NAs are also present in other biological systems, for example bacteria, and these non-influenza NAs are critical virulence factors in many pathogenic organisms including Streptococcus pneumoniae, Pseudomonas aeruginosa, and Vibrio cholerae. The viral enzyme is a mushroom-like shaped homotetramer, while the bacterial NA is a monomer with two flanking lectin-like domains. Both enzymes share the canonical six-blade β-propeller fold of the catalytic NA domain, despite exhibiting a relatively low amino acid sequence identity of only 12% as revealed by structure-based sequence alignment. Instead, we solved the crystal structures of bacterial VCNA in complex with the reference compounds oseltamivir carboxylate and zanamivir at 1.87 and 1.75 Å resolution, allowing a comparative analysis of bacterial versus viral enzyme-inhibitor interactions for these synthetic substances.

The bacterial VCNA, on the other hand, is only moderately inhibited by the reference compounds, displaying IC50 values of 144 µM for oseltamivir carboxylate and 52 µM for zanamivir. A common feature of viral and bacterial inhibitor binding is the electrostatic and hydrogen bonding interaction of the carboxylic acid group of oseltamivir carboxylate or zanamivir to a cluster of three positionally conserved arginine residues (Arg224, Arg635, and Arg712 in VCNA; Arg118, Arg292, and Arg371 in H1N1-NA). A second common structural feature is the electrostatic and hydrogen bonding interaction of the 5-amino group of oseltamivir carboxylate or the 4-guanidino moiety of zanamivir with an electronegative binding pocket within the active site (Glu243, Arg 245, Asp250 and Asp292 in VCNA; Glu119, Asp151, and Glu227 in H1N1-NA). Moreover, the acetamido binding cavity in bacterial VCNA is sterically constrained by the short amino acid stretch of Gln317 and Asn318 that extends into the active site. Another steric restriction in the bacterial VCNA active site is seen in the microenvironment around the 5-amino group of oseltamivir carboxylate and the 4-guanidino moiety of zanamivir. Glu243 and Arg245 extend further into the active site compared to Leu134 and Arg156 of the influenza enzyme, thereby reducing the available space in that subpocket. To rationalize the observed increased inhibitory activity of zanamivir over oseltamivir carboxylate for bacterial VCNA (IC50 of 52 µM versus 144 µM), we compared the inhibitor interactions in the determined VCNA complex structures. The 4-guanidino group of zanamivir, for example, forms electrostatic and hydrogen bonding interactions with Glu243, Arg245, and Asp292, whereas the 5-amino group of oseltamivir carboxylate interacts with Arg250 only. The hydrophilic 6-(1′,2′,3′)-trihydroxypropyl group of zanamivir hydrogen bonds with Asn318 and Asp637, the corresponding 3-(1′-ethylpropoxy) group of oseltamivir carboxylate, however, interacts only hydrophobically.

> ALFDYNATGDTEFDSPAKQGWMQDNTNNGSGVLTNADGMPAWLVQGIGGRAQWTYSLSTNQHAQASSFGWRMTTEMKVLSGGMITNYYANGTQRVLPIISLDSSGNLVVEFEGQTGRTVLATGTAATEYHKFELVFLPGSNPSASFYFDGKLIRDNIQPTASKQNMIVWGNGSSNTDGVAAYRDIKFEIQGDVIFRGPDRIPSIVASSVTPGVVTAFAEKRVGGGDPGALSNTNDIITRTSRDGGITWDTELNLTEQINVSDEFDFSDPRPIYDPSSNTVLVSYARWPTDAAQNGDRIKPWMPNGIFYSVYDVASGNWQAPIDVTDQVKERSFQIAGWGGSELYRRNTSLNSQQDWQSNAKIRIVDGAANQIQVADGSRKYVVTLSIDESGGLVANLNGVSAPIILQSEHAKVHSFHDYELQYSALNHTTTLFVDGQQITTWAGEVSQENNIQFGNADAQIDGRLHVQKIVLTQQGHNLVEFDAFYLAQQTPEVEKDLEKLGWTKIKTGNTMSLYGNASVNPGPGHGITLTRQQNISGSQNGRLIYPAIVLDRFFLNVMSIYSDDGGSNWQTGSTLPIPFRWKSSSILETLEPSEADMVELQNGDLLLTARLDFNQIVNGVNYSPRQQFLSKDGGITWSLLEANNANVFSNISTGTVDASITRFEQSDGSHFLLFTNPQGNPAGTNGRQNLGLWFSFDEGVTWKGPIQLVNGASAYSDIYQLDSENAIVIVETDNSNMRILRMPITLLKQKLTLSQN> MRGSHHHHHHGSSTVDEL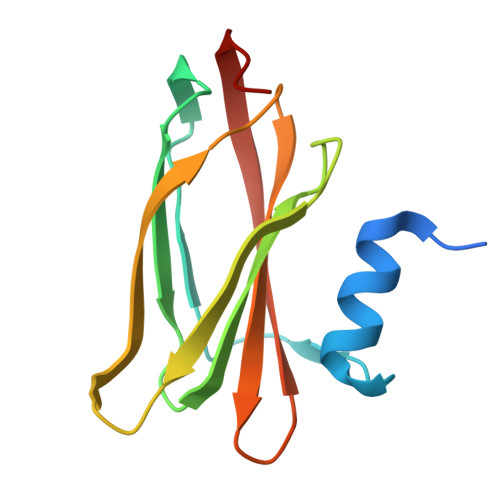TAAFTGGAATGEGGLTLTAPEIAENGNTVPIEVKAPGAVAIMLLAAGNPEPAVATFNFGPAAADQRAATRIRLAQTQDVIALAKMADGSVVKAQTTVKVTIGGCGG> ANIVGGIEYSINNASLCSVGFSVTRGATKGFVTAGHCGTVNATARIGGAVVGTFAARVFPGNDAAWVSLTSAQTLLPRVANGSSFVTVRG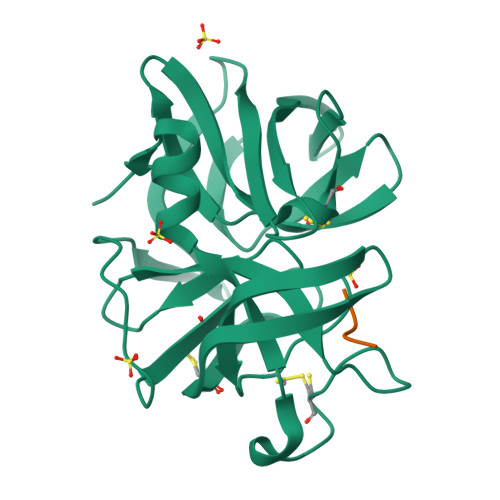STEAAVGAAVCRSGRTTGYQCGTITAKNVTANYAEGAVRGLTQGNACMGRGDSGGSWITSAGQAQGVMSGGNVQSNGNNCGIPASQRSSLFQRLQPILSQYGLSLVTG;> LQPI>[2x]MGAEEEDTAILYPFTISGNDRNGNFTINFKGTPNS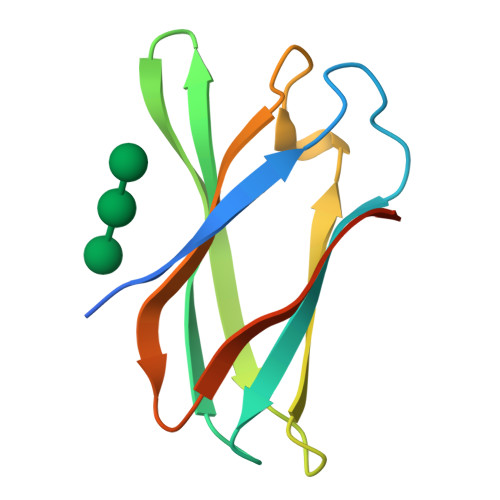TNNGCIGYSYNGDWEKIEWEGSCDGNGNLVVEVPMSKIPAGVTSGEIQIWAHSGDLKMTDYKALEHHHHHH>[2x]GIDPFTMKYVGSIDQGTTSTRFIIFDERQRPVSVHQVPHTQHTPHPGWLEHDPMEIFRSACKCMSVAIAKLRQKDASFRKIEAIGITNQRETTVAWDRVTKEPLCYAPVWNDLRTYDITKKVTAELGGGDSMFASKITGLPVSTYFAAFKMRWMLENVPAVADACRRGTLCFGTIDTWLMYKLSGGKAFVTDVTNA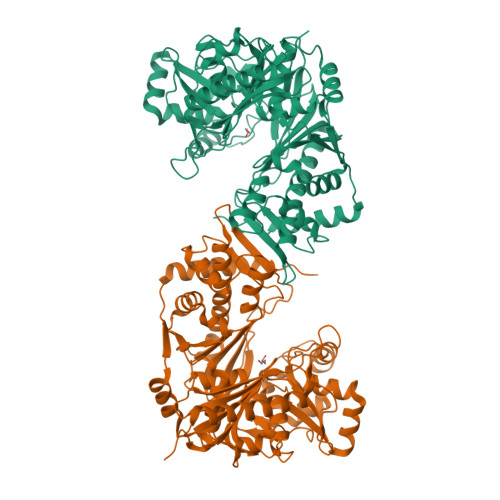SRTFLMDLRTRKWSPELCEKLKIPMETLPEIRSNSELFGYVETDECGVAAALNERTPIMGSIGDQQSALFGNMCFEKGEAKNTYGTGCFLLMNVGEEARFSKHGLLSTVGFQVGRDGPCYYALEGAIACAGATVEWMRRNMNLFSHITECEKLARSVPGTQGIVFVPAFSGLLAPYWDPSARGTIVGMTLKTTRAHVIRAALQAIALQLNDVVGSMKRDAGLNLSSLRVDGGLSKNGLLMEIQASLLGVDILVPSMHETTALGAALCAGLAAGVWTSLEEVKAVSRRENSWKTVSPSGSAMEREAMIAEWREALKRTKWAKL> MSMLKREDWYDLTRTTNWTPKYVTENELFPEEMSGARGISMEAWEKYDEPYKITYPEYVSIQREKDSGAYSIKAALERDGFVDRADPGWVSTMQLHFGAIALEEYAASTAEARMARFAKAPGNRNMATFGMMDENRHGQIQLYFPYANVKRSRKWDWAHKAIHTNEWAAIAARSFWDDMMMTRDSVAVSIMLTFAFETGFSNMQFLGLAADAAEAGDHTFASLISSIQTDESRHAQQGGPSLKILVENGKKDEAQQMVDVAIWRSWKLFSVLTGPIMDYYTPLESRNQSFKEFMLEWIVAQFERQLLDLGLDKPWYWDQFMQDLDETHHGMHLGVWYWRPTVWWDPAAGVSPEEREWLEEKYPGWNDTWGQCWDVITDNLVNGKPELTVPETLPTICN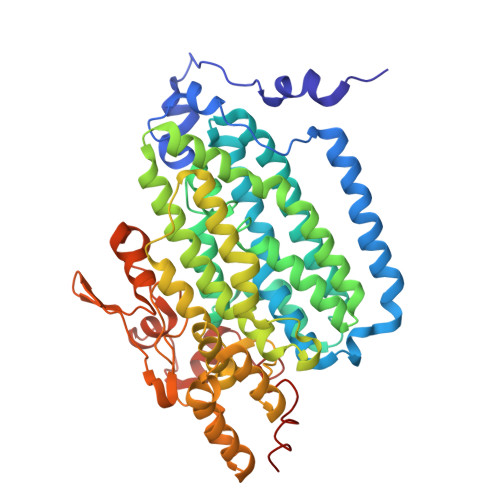MCNLPIAHTPGNKWNVKDYQLEYEGRLYHFGSEADRWCFQIDPERYKNHTNLVDRFLKGEIQPADLAGALMYMSLEPGVMGDDAHDYEWVKAYQKKTNAA>MTKQEKTALNMARFIRSQTLTLLEKLNELDADEQADICESLH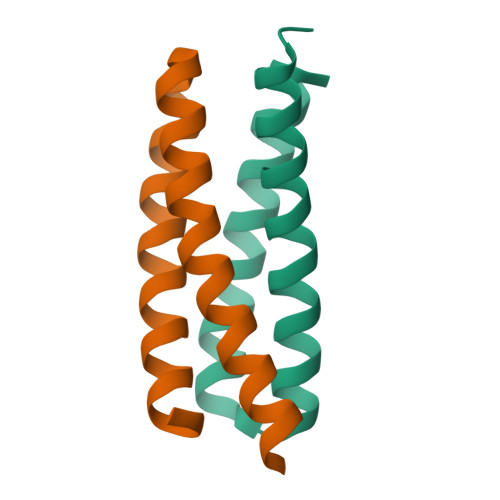DHADELYRSCLARFGDDGENL[2x]> SMCNPSACRAVGRGLQPKGVRVKETADFKVYTKGAGSGELKVTVKGPKGEERVKQKDLGDGVYGFEYYPMVPGTYIVTITWGGQNIGRSPFEVKVGTECGNQKVRAWGPGLEGGVVGKSADFVVEAIGDDVGTLGFSVEGPSQAKIECDDKGDGSCDVRYWQQEAGEYAVHVLCNSEDIRLSPFMADIRDAPQDFHPDRVKARGPGLEKTGVAVNK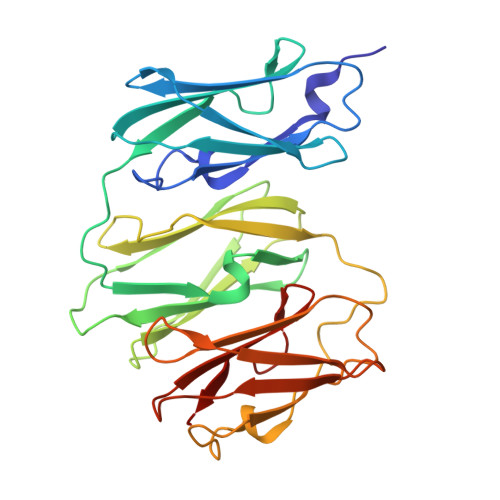PAEFTVDAKHGGKAPLRVQVQDNEGCPVEALVKDNGNGTYSCSYVPRKPVKHTAMVSWGGVSIPNSPFRVNVGAG> SALFEPYTLKDVTLRNRIAIPPMCQYMAEDGMINDWHHVHLAGLARGGAGLLVVEATAVAPEGRITPGCAGIWSDAHAQAFVPVVQAIKAAGSVPGIQIAHAGRKASANRPWEGDDHIAADDTRGWETIAPSAIAFGAHLPKVPREMTLDDIARVKQDFVDAARRARDAGFEWIELHFAHGFLGQSFFSEHSNKRTDAYGGSFDNRSRFLLETLAAVREVWPENLPL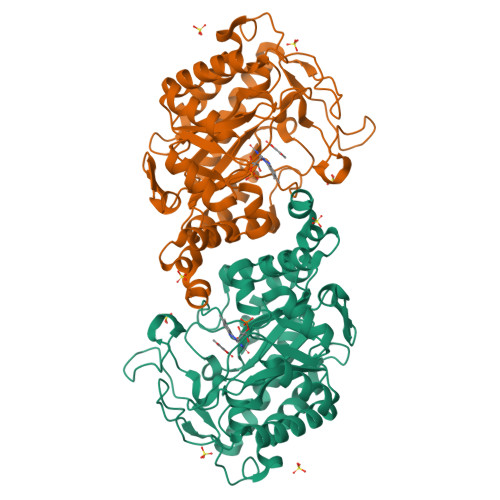TARFGVLEYDGRDEQTLEESIELARRFKAGGLDLLSVSVGFTIPDTNIPWGPAFMGPIAERVRREAKLPVTSAWGFGTPQLAEAALQANQLDLVSVGRAHLADPHWAYFAAKELGVEKASWTLPAPYAHWLER>QLLGLLGQAATVIGGEPTVSVEQLDFSAARGDVALQVRAPGFDVLERLRSRLSESGLAVQLGSASRDGSTVSARLVIG[2x]

In our studies we have focused on the periplasmic segment of GspL (historically called XcpY) from P. aeruginosa, GspLperi, which consists of two domains: a membrane proximal domain (MPD) connected via a short linker to a ferredoxin-like domain (FLD). The inner-membrane bitopic protein GspL can be considered a central player in the T2SS because it appears to interact extensively with other components of the system. Even though the exact mode of secretion via T2SS has not been fully elucidated, the role of GspL is anticipated to help in linking adenosine triphosphate (ATP) hydrolysis to the assembly of the pseudopilus, which together constitute the two crucial steps in exoprotein transport. In this work we presented two distinct crystal structures of GspLfld, which in combination with the crystal structure of GspLfld from Vibrio parahaemolyticus, provide direct evidence for the conservation of a hydrophobic dimer interface.

In contrast to the dimer of GspLfld in crystal form 1 and the dimer of GspLfld from V. parahaemolyticus, crystal form 2 displays a full dimer in the crystal asymmetric unit. The different inter-strand distances between β1 and β1′ in P. aeruginosa GspLfld crystal forms result in two distinct conformations of the GspLfld dimer. The distance between the main chain atoms of β1 and β1′ of crystal form 1 is in the range of 4.5–5.0 Å and is drastically greater than the equivalent interdomain in crystal form 2, which are instead within hydrogen bonding distances (2.8–3.0 Å). In this regard, crystal form 2 and the V. parahaemolyticus crystal form of GspLfld appear as closed versions of the dimer whereas crystal form 1 exploits a novel conformation, resulting in an open variant of the interface. Notwithstanding complementation of the hydrophobic interface by extension of antiparallel β-sheet over two ferredoxin-like domains in cases of crystal form 2 and V. parahaemolyticus dimeric structure, crystal form 1 have adapted the open variant of dimer. A more indirect hint came from the necessity to model the two dimer interface residues Leu327 and Phe329 into two conformations for each residue, in crystal forms 1 and 2, respectively.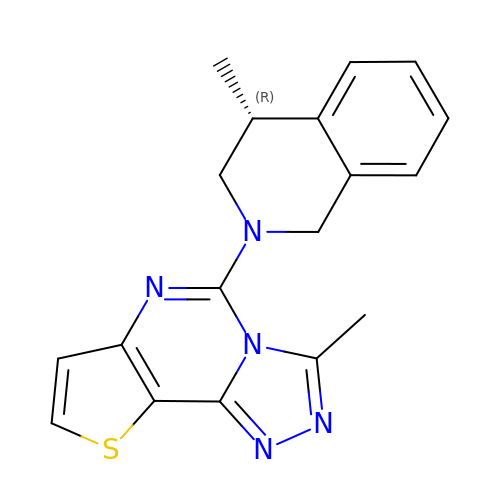(4R)-3-methyl-5-[(4R)-4-methyl-3,4-dihydroisoquinolin-2(1H)-yl]thieno[2,3-e][1,2,4]triazolo[4,3-c]pyrimidine | C18 H17 N5 S | GGQQENQZNLSCPW-NSHDSACASA-N>SNAQHTTIGDVLREHRRSHPGRTALVDGPVRLTWPELDDRVNRLAGSLAASGIGRGDRIMWLGQNSFRVYELIAAAGKLGAMVCVGYWRWAPPEMEFALRDFDPHLVVWQHQEIHETVARTREALGSDDTARWLRHDSAPQDPDGYEAFLAAGGLADPDLDIDPDSPVLVLYTAAMSGRQCGSLLSHTNLIAMATAAAWLGDIDHTTAFLNSGPMFHIGNHQFWGMPTLLMAGKNVIVRRVVAEEVRDLLVAEECTHAFLMPPTVAEIVRLNRDTGHDLSRLRATVAPHLWEGMATTDTSRFTRSGAAAGRGYGQTELSGFAVTAAYGGPAAGNAGRPGPGLTVRVLDTAGRECAVGEAGEICARGTVVHRGYWNRDEVNAHRFRSGWWHTTDLGRREPDGSLTFLGTTTRMLKSAAENIFPAEVENCIEQHPAVREAAVIGVPNTRWAQDVKAVVVLEPDAGVSEQEIIDHCRPRIASYKKPKSVAFA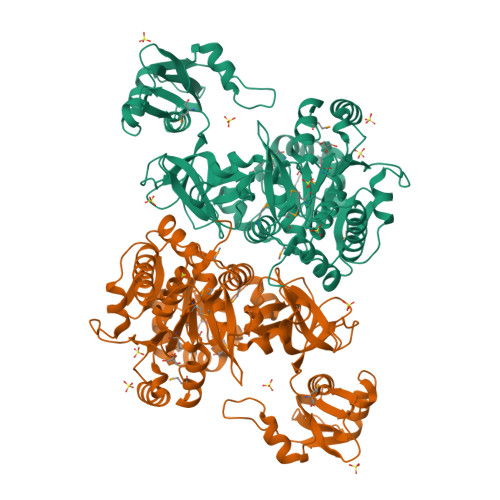AALPRTVSGARDYDALDKEYGGGGYPGAATLGPGR[2x]> MAPLVDNPQIKSAELLRPLPLYQHAYVWPYVIVWPVFLRVYLTQELYDKYIGAQEWTFVWIISIVTFQTLTWLCTHWSVNLNALFTAKKASSIEDAQLIKVIPVANAGAADICKLVRDKVGDNKTNISFLFQKRRFLWYPERKAFSTLEFDIDAEPKPTLSKFQLSRGIESEDELKRLEQHYGTNTFDIPVPTFTELFKEHAVAPF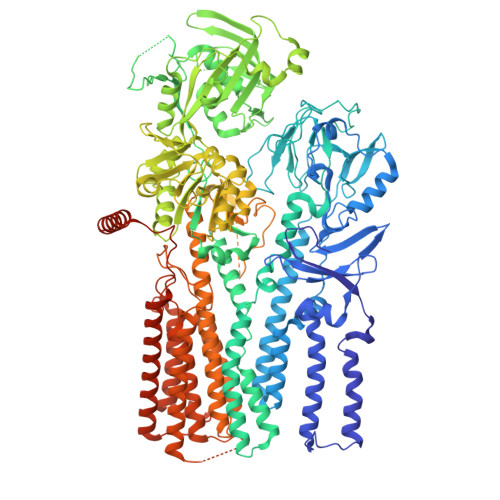FVFQVFCVGLWLLDEYWYYSLFTLVMLVVFESTVVWQRQRTLTEFRSMSIKPYPIYVYRLGKWTEIQSDKLLPGDLVSVTRTKEDSGVACDMILVEGTAIVNEAMLSGESTPLLKDSIQLRPGDAVLEVDGLDKNSLLWGGTKVLQITHGTAEEERPKPASGIPPPPDNGAMAVVTKTGFETSQGSLVRTMIYSTERVSANNTEALLFILFLLVFALAASWYVWDEGVRKDRKRSKLLLDCILIITSVVPPELPMELSLAVNTSLSALAKFAIFCTEPFRIPFAGRIDVACFDKTGTLTGEDLVVEGIAGLGLGHSGTDTPKEADGAHTRMVSVHDAGMETTLVLATAHALVKLDEGEIVGDPMEKATLNALGWVLGKNDTLTSKPGNAASSGILGTVQIKRRFQFSSALKRQSSVATITATEVKTGRKLRGSFVGVKGAPETIMKMLVTVPEHYEETYKYFTRRGSRVLALAYKQLTTEGELGANKINDLKRESVEADLHFAGFLVLQCPLKEDAKQAVRMLNESSHRVVMITGDNPLTAVHVAKEVEIVDRDVLILDAPEHSVYGEESLVWRSVDDKIRIDVDPTKPIDPEILKTKDLCVTGYALNKFKGQVGWKSLLRYTWVYARVSPKQKEDILLGLKDMGYYTLMAGDGTNDVGALKQAHVGVALLNGTQEDLNRIAEHTRNQKMKELYQKQVDLMARWGQPPPPVPAMIAHLYPPGPSNPHYQKAMEREAQKRGVTVEQLAKVNGTNVTSNPAGVQQQSGQDAKKAKQVEAAKKAANFADKLTSSLMEAEMDDEPPTLKLGDASVAAPFTSKLRNVMAIPNILRQGRCTLVATIQMYKILALNCLISAYSLSVLYLEGIKFGDGQITISGMLMSVCFLSISRARSVEGLSKERPQPNIFNFYIIGSILGQFAVHVATLIYIAQLCDQIEPRTEVIDLEAEFKPSLLNSAVYLLQLIQQISTFAVNYQGRPFRESLSENKGMFYGIVGVTAIAFACSTEMLPELNEAMKLVPFNENFKTIMTTVMIIDFVACYVIEWVLKKLFSDLRARDIAERRPDQLERERVRKEKEAREKEEEEERKERERIEAFERRLEEKRTRLVEAAAQREQQQQQWAQRR> ACRQEPQPQGPPPAAGAVASYDYLVIGGGSGGLASARRAAELGARAAVVESHKLGGTCVNVGCVPKKVMWNTAVHSEFMHDHADYGFPSCEGKFNWRVIKEKRDAYVSRLNAIYQNNLTKSHIEIIRGHAAFTSDPKPTIEVSGKKYTAPHILIATGGMPSTPHESQIPGASLGITSDGFFQLEELPGRSVIVGAGYIAVEMAGILSALGSKTSLMIRHDKVLRSFDSMISTNCTEELENAGVEVLKFSQVKEVKKTLSGLEVSMVTAVPGRLPVMTMIPDVDCLLWAIGRVPNTKDLSLNKLGIQTDDKGHIIVDEFQNTNVKGIYAVGDVCGKALLTPVAIAAGRKLAHRLFEYKEDSKLDYNNIPTVVFSHPPIGTVGLTEDEAIHKYGIENVKTYSTSFTPMYHAVTKRKTKCVMKMVCANKEEKVVGIHMQGLGCDEMLQGFAVAVKM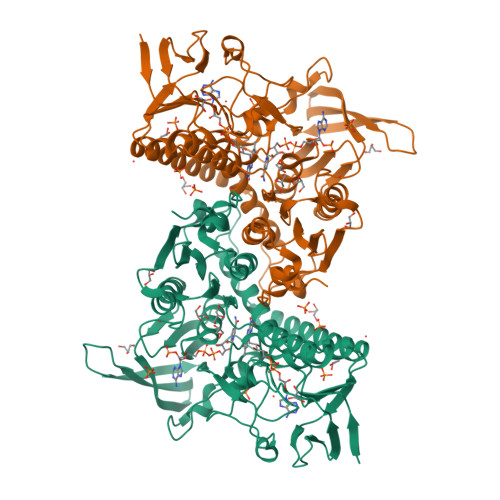GATKADFDNTVAIHPTSSEELVTLR>MAHHHHHHAALRQPQVAELLAEARRAFREEFGAEPELAVSAPGRVNLIGEHTDYNQGLVLPMALELMTVLVGSPR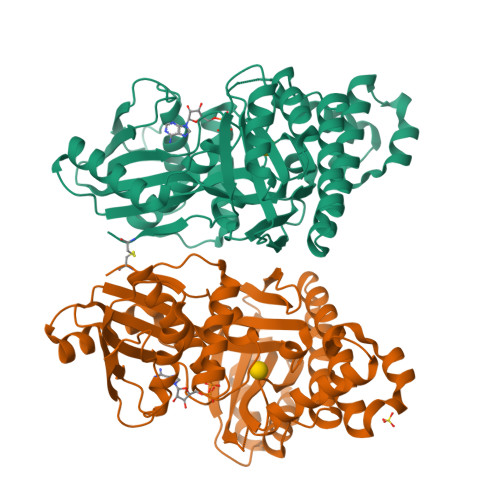KDGLVSLLTTSEGADEPQRLQFPLPTAQRSLEPGTPRWANYVKGVIQYYPAAPLPGFSAVVVSSVPLGGGLSSSASLEVATYTFLQQLCPDSGTIAARAQVCQQAEHSFAGMPCGIMDQFISLMGQKGHALLIDCRSLETSLVPLSDPKLAVLITNSNVRHSLASSEYPVRRRQCEEVARALGAASLREVQLEELEAARDLVSKEGFRRARHVVGEIRRTAQAAAALRRGDYRAFGRLMVESHRSLRDDYEVSCPELDQLVEAALAVPGVYGSRMTGGGFGGCTVTLLEASAAPHAMRHIQEHYGGTATFYLSQAADGAKVLCL[8x]TLKs belong to a distinct branch of Ser/Thr kinases, that appear to be constitutively expressed in most cell lines and tissues, and they exhibit the highest levels of activity during S-phase. Human TLK1 and TLK2 polypeptides are composed of an N-terminal region, a middle region of helices predicted to contain three coiled coils (CC) and a C-terminal kinase domain that shows 94% identity between TLK1 and TLK2. The precise mechanisms by which ASF1 is regulated remain unclear, but ASF1 was identified as a target of the Tousled kinase (TSL) and Tousled-like kinases (TLKs) that can influence its stability and histone binding capacity. Our biochemical analysis has identified key autophosphorylation sites critical for its activity and indicates that TLK2 is activated through a cis-autophosphorylation mechanism.

The divergent sequence conservation of the catalytic domain of TLK2, when compared to other kinases, is reflected in its structure. Our unphosphorylated ATPγS TLK2 structure is in a pre-active conformation. Although the R-spine is in the correct alignment to create a platform for an active conformation, important hallmarks of the active state, such as the salt bridge between the conserved lysine and glutamate in the β3 and αC helix (K491 and E514 in TLK2) are not observed. However, TLK2 does not contain this motif, a Tyr residue is located in the Arg position, suggesting that TLKs may not need T-loop phosphorylation for activation. Out of the 15 phosphosites, we can locate nine of them in the structure of the kinase domain, mainly in the C-lobe, around the catalytic and activation loops. Unfortunately, we cannot observe the residues phosphorylated in the C-tail (T750 to S771) because this region was not included in our crystallized protein. The modelling of a phosphoserine instead of S474 in the P-loop of the kinase domain suggests that this modification could affect nucleotide binding, leading to a reduction in activity. The H518R mutation is located on the bottom of αC-helix and is conserved in other kinases, constituting the RS3 of the regulatory spine.

> MGSSHHHHHHSTGSTEHSCSSQKQISIQHRQTQSDLTIEKISALENSKNSDLEKKEGRIDDLLRANCDLRRQIDEQQKMLEKYKERLNRCVTMSKKLLIEKSKQEKMACRDKSMQDRLRLGHFTTVRHGASFTEQWTDGYAFQNLIKQQERINSQREEIERQRKMLAKRKPPAMGQAPPATNEQKQRKSKTNGAENETPSSGNTELKDTAPALGAHSLLRLTLAEYHEQEEIFKLRLGHLKKEEAEIQAELERLERVRNLHIRELKRIHNEDNSQFKDHPTLNDRYLLLHLLGRGGFSEVYKAFDLTEQRYVAVKIHQLNKNWRDEKKENYHKHACREYRIHKELDHPRIVKLYDYFSLDTDSFCTVLEYCEGNDLDFYLKQHKLMSEKEARSIIMQIVNALKYLNEIKPPIIHYDLKPGNILLVNGTACGEIKITDFGLSKIMDDDSYNSVDGMELTSQGAGTYWYLPPECFVVGKEPPKISNKVDVWSVGVIFYQCLYGRKPFGHNQSQQDILQENTILKATEVQFPPKPVVTPEAKAFIRRCLAYRKEDRIDVQQLACDPYLLPHIRKSVSTSSPA>[8x]NATGA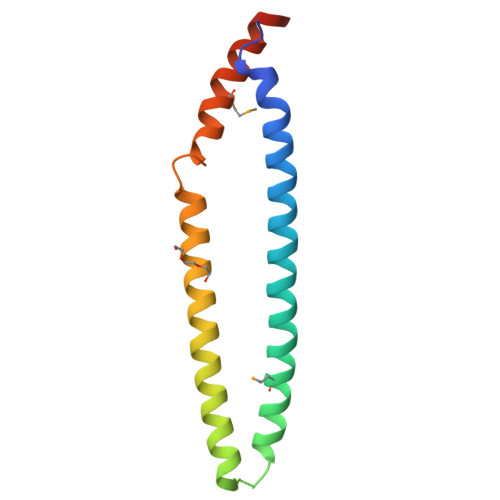ISNLIPKLGELLTEEFKLHKGVKKNIEDLGKELESMNAALIKIGEVPREQLDSQDKLWADEVRELSYVIEDVVDKFLVQVDGIKSDDNNNKFKGLMKRTTELLKKVKHKHGIA2',3'-O-[(1R,6R)-2,4,6-trinitrocyclohexa-2,4-diene-1,1-diyl]adenosine 5'-(trihydrogen diphosphate) | C16 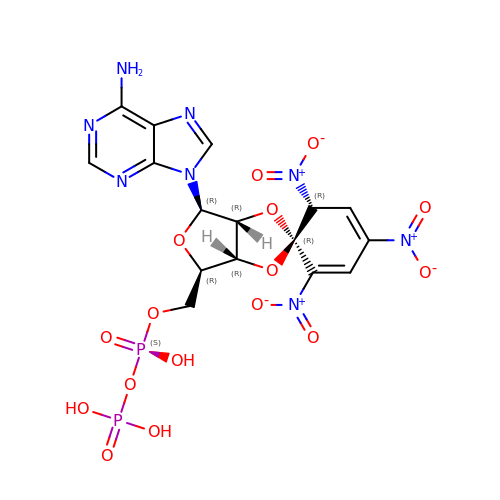H16 N8 O16 P2 | WYOHYTDXVJMKHS-BENPRDFYSA-N> MHHHHHHTRPDSKSMNYQLLKTFSRQPIQFGRFLARLLAGLVNTLKITRTSKSIELN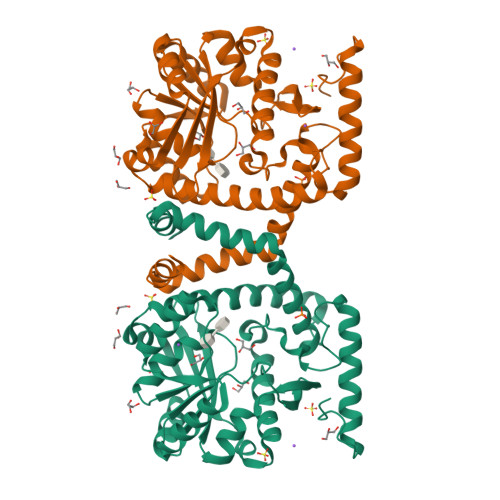LRIALPYLTPQQRIAITEKAVRNELTSYFEFLSIWGSSNSKNISRIHRIEGEHFFHEALAAKKGVVLIVPHFGTWEVMNAWCAQFTSMTILYKPVKNADADRFVREARSREQANLVPTDESGVRQIFKALKQGETTVILPDHTPNVGGDMVNYFGVPLASSNLSAKLIQKTKAKALFLYAIRNENDGFTMHIEPMDEKIYEGTADDGTYVIHQAIEQLIYQYPEHYHWSYKRFKANPALDNIYNIDPTEALKIVDRLKAEALKTSTQPEPIQTSVM Recently, a shortened Dscam (sDscam) gene family with tandemly arrayed 5′ cassettes in Chelicerata species has been identified, which encodes ∼50–100 isoforms. Chelicerata sDscams could be classified into two subfamilies, sDscamα and sDscamβ, containing one and two variable Ig domains, respectively. Crystal structures and cell aggregation assays demonstrated that both α and β subfamilies of sDscam used Ig1 for the isoform-specific trans recognition in a hand-in-hand manner. Furthermore, the cis interactions were established by the three FNIII domains of sDscam, which assemble into a cross fold with a kink between FNIII2 and FNIII3.

We also determined the crystal structures of sDscam Ig1 from another chelicerate species Limulus polyphemus (isoforms α7 and β3v7) to provide insights into the conservation of sDscam trans recognition within Chelicerata. These crystal structures of Ig fragments were determined at 1.3–3.1 Å resolutions. The crystal structures of sDscam Ig1 from both M. martensii and L. polyphemus revealed a common assembly of antiparallel homodimer for both α and β subfamilies of sDscam. In addition, all these Ig1 homodimers resemble each other well with root mean square deviation (RMSD) values of 1.0–1.6 Å, indicating a shared mechanism of sDscam trans recognition within Chelicerata. Similarly, sDscam Ig1 also employs the ABED face to form an antiparallel homodimer. However, among the seven Ig1 structures reported here, the complementary electrostatic potential surface pattern (negative in one end, neutral in the middle, and positive in the other end) has been only observed in the three β isoforms, but not in any one of the four α isoforms. Structural analysis showed that B and E strands constituted the core of ABED face and dominated the trans homophilic interactions of sDscam Ig1. Electrostatic and shape complementarity had been observed in all Ig1 dimer interfaces. The electrostatic repulsion and/or shape non-complementarity may avoid the binding between different sDscam isoforms, resulting in isoform-specific interactions.

> GASGSDFPVISPFTFPTNVRLGEQVRVFCTVRRGNPPFSFAWFKEGEKLITGQHIEVENTDKYTSKLGILNVSTLDIGNYTCEITNQDGKDSATSRLIVEAP> MYIQVLGSAAGGGFPQWNCNCVNCKGYRDGTLKATARTQSSIALSDDGVHWILCNASPDIRAQLQAFAPMQPARALRDTGINAIVLLDSQIDHTTGLLSLREGCPHQVWCTDMVHQDLTTGFPLFNMLSHWNGGL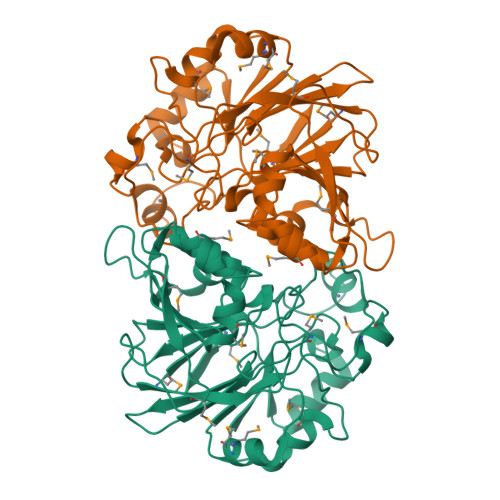QWNRIELEGSFVIDACPNLKFTPFPLRSAAPPYSPHRFDPHPGDNLGLMVEDTRTGGKLFYAPGLGQVDEKLLAMMHGADCLLVDGTLWEDDEMQRRGVGTRTGREMGHLAQNGPGGMLEVLDGFPRQRKVLIHINNTNPILDENSPERAEVLRRGVEVAFDGMSIELLEHHHHHH6,6,8-trimethyl-5,6-dihydro[1,3]dioxolo[4,5-g]quinoline | C13 H15 N O2 | 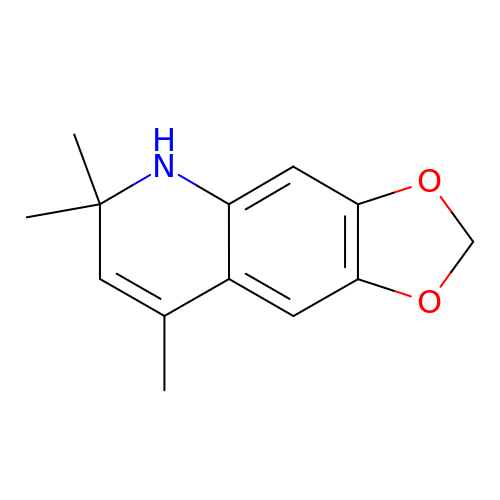JAMOHNXWLCCTQU-UHFFFAOYSA-N2-(2-phenoxypyridin-3-yl)[1,3]thiazolo[5,4-c]pyridine 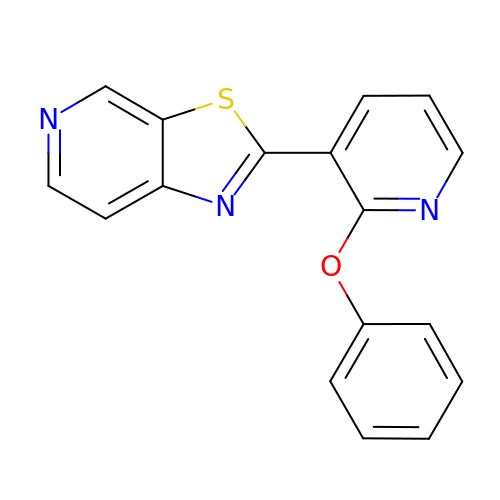| C17 H11 N3 O S | BEFVRNYCLDLVCZ-UHFFFAOYSA-N> ECVTQLLKDTCFEGGDITTVFTPSAKYCQVVCTYHPRCLLFTFTAESPSEDPTRWFTCVLKDSVTETLPRVNRTAAISGYSFKQCSHQISACNKDIYVDLDMKGINYNSSVAKSAQECQERCTDDVHCHFFTYATRQFPSLEHRNICLLKHTQTGT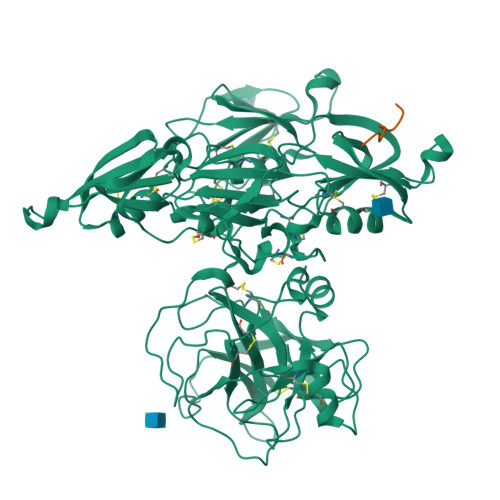PTRITKLDKVVSGFSLKSCALSNLACIRDIFPNTVFADSNIDSVMAPDAFVCGRICTHHPGCLFFTFFSQEWPKESQRNLCLLKTSESGLPSTRIKKSKALSGFSLQSCRHSIPVFCHSSFYHDTDFLGEELDIVAAKSHEACQKLCTNAVRCQFFTYTPAQASCNEGKGKCYLKLSSNGSPTKILHGRGGISGYTLRLCKMDNECTTKIKPRIVGGTASVRGEWPWQVTLHTTSPTQRHLCGGSIIGNQWILTAAHCFYGVESPKILRVYSGILNQSEIKEDTSFFGVQEIIIHDQYKMAESGYDIALLKLETTVNYTDSQRPICLPSKGDRNVIYTDCWVTGWGYRKLRDKIQNTLQKAKIPLVTNEECQKRYRGHKITHKMICAGYREGGKDACKGDSGGPLSCKHNEVWHLVGITSWGEGCAQRERPGVYTNVVEYVDWILEKTQAV;> NPISDFPD>MQTLIIVAHPELARSNTQPFFKAAIENFSNVTWHPLVADFNVEQEQSLLLQNDRIILEFPLYWYSAPALLKQWMDTVMTTKFATGHQYALEGKELGIVVSTGDNGNAFQAGAAEKFTISELMRPFEAFANKTKMMYLPILAVHQFLYLEPDAQQRLLVAYQQYATNVGALEHHHHHH[2x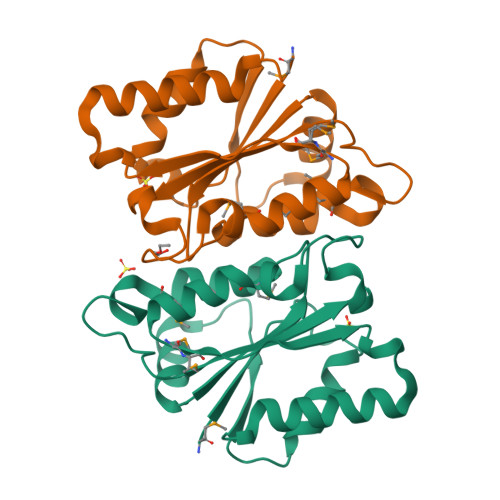]6-bromanyl-~{N}-[[(1~{S},2~{S})-2-chloranylcyclohexyl]methyl]-1~{H}-indazol-4-amine | C14 H17 Br Cl N3 | 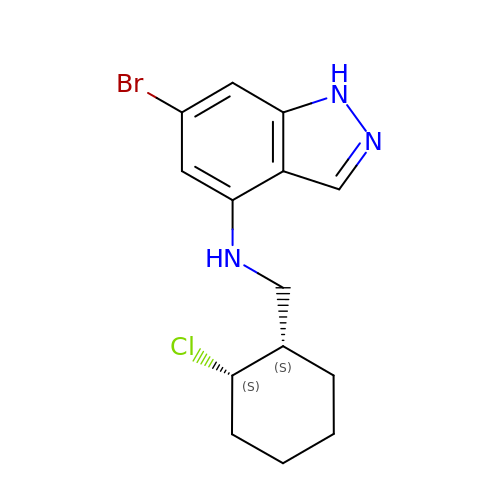BLJSKYLBFPXWFR-CABZTGNLSA-N>[2x]GAMGSGLAKYLPSTIKLVSKSGTVSPISLAGKTVFFYFSASWCPPCRGFTPTLVEFYEKFRESKNFEVVLVTWDDEEEAYNGYFAKMP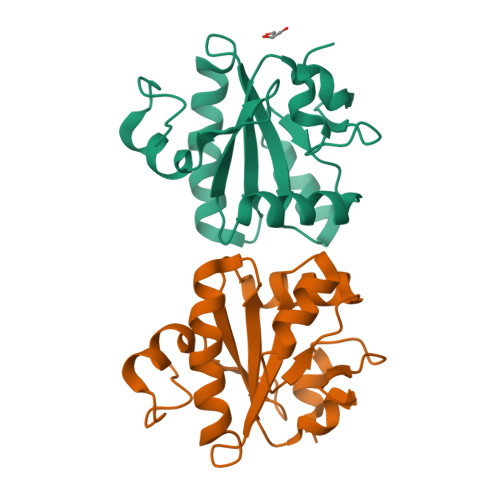WLAIPFSSRAELEALRSTFGVETIPTVIAVNADTGAVVSTKGRERLLTDPEGKNFPWSD> MPSTDSIPKSNFDAIPDVIQAFKNGEFVVVLDDPSRENEADLIIAAESVTTEQMAFMVRHSSGLICAPLTPERTTALDLPQMVTHNADPRGTAYTVSVDAEHPSTTTGISAHDRALACRMLAAPDAQPSHFRRPGHVFPLRAVAGGVRARRGHTEAGVELCRLAGKRPVAVISEIVDDGQEVEGRAVRAAPGMLRGDECV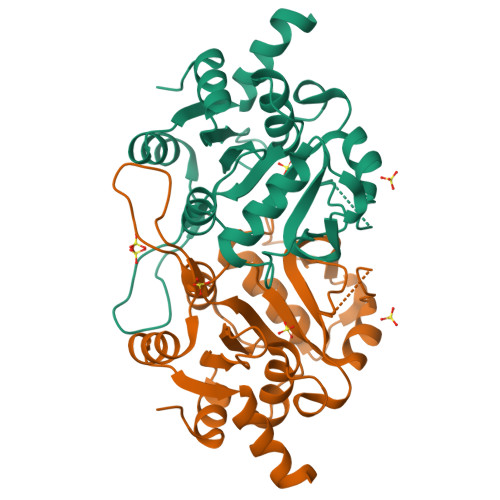AFARRWGLKVCTIEDMIAHVEKTEGKLETNGSG2-METHYL-N-PHENYL-5,6-DIHYDRO-1,4-OXATHIINE-3-CARBOXAMIDE 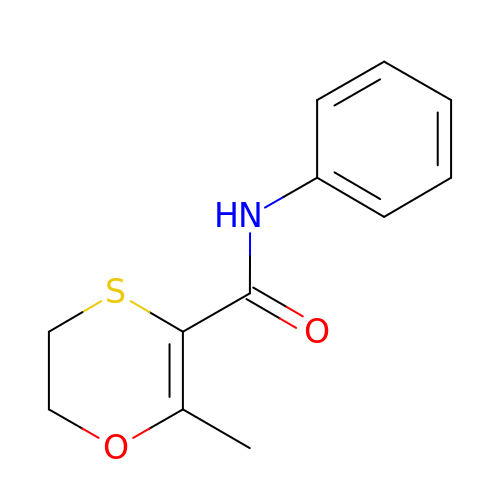| C12 H13 N O2 S | GYSSRZJIHXQEHQ-UHFFFAOYSA-N> MLICNFLMYSNFSRIYWFDFNGTVNENLPLNYNVLKICRNEINKLEKLNENNLGTQKNPIKLNLSFEDKHYNTNNLVLDLNSYETFNSKNFISSIFDKTFESLNTVLMAPIYSFLEFKLKLSSTKINTNHYYVINGKLYITYNDSFKLFTTINDYFNDLNELSNTKLFFLYRSFNIYNIKLNSLVDFVFLKLILFIHLLYLKSTNYNRFDYRLKQTDWGFYINNNSNYIQNIFSGLKYIWRGLRFWIIGLLLGLSSIYYLMYVRLLPFNKIIFAWILVAMFLYWLLSGFVFFVKKYQYSKFTAAIQRFWKRTYIIFW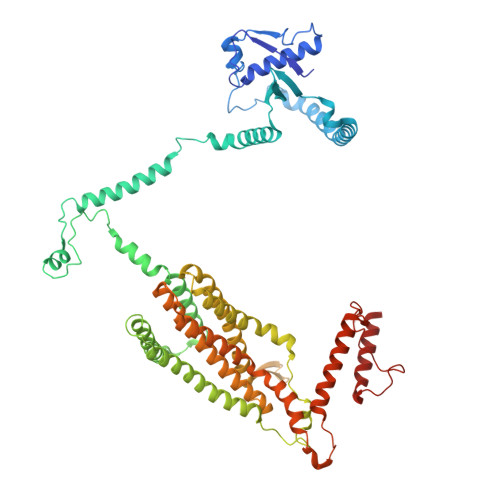VIEAGTFSVFFYLTLNASSEPVYMYDQIKIYKTHLFSWRWFLIKLLPSVSIILLGYYLQLTLKWNLFNKQNTIVLLITLLLLYILWLEFYQFYHILSFYGNINWAFDYDEYIWTLELDTRRTRLANNYIAICLFAKFWHFVFIFLFWVFFVLRINELGRIRYPLLVANVQNFIIIYIMSWAYMYPWLKFIFRKYLDVPYYWFYLNGRELGIRVFFTDLKLFFYGITNRLFDFNPSSIKFEKYPFYYWINSSQLTEFNQYRKFVIRDSIIYSLNNYII> ADPLPLPEVQCFVFNV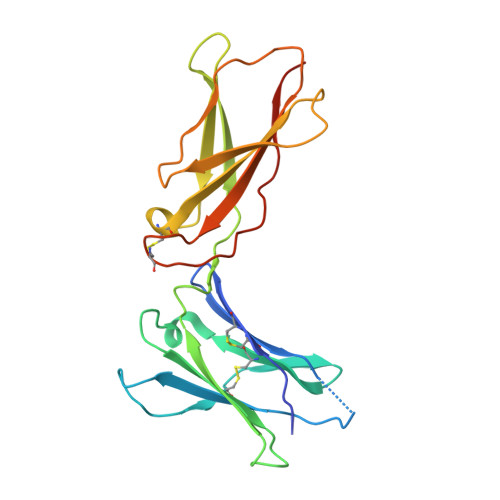EYMNCTWQSSSEPQPTNLTLHYWYKNSDNDKVQKCSHYLFSEEITSGCQLQKKEIHLYQTFVVQLQDPREPRRQATQMLKLQNLVIPWAPENLTLHKLSESQLELNWNNRFLNHCLEHLVQYRTDWDHSWTEQSVDYRHKFSLPSVDGQKRYTFRVRSRFNPLCGSAQHWSEWSHPIHWGSNTSKEN> MVERTA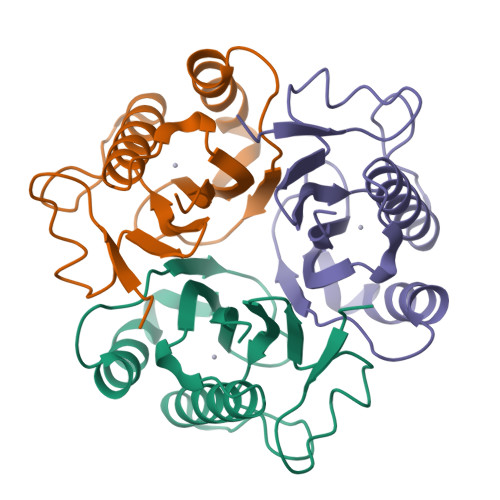VFPAGRHSLYAEHRYSAAIRSGDLLFVSGQVGSREDGTPEPDFQQQVRLAFDNLHATLAAAGCTFDDIIDVTSFHTDPENQFEDIMTVKNEIFSAPPYPNWTAVGVTWLAGFDFEIKVIARIPEQ2-(3,4-dimethoxyphenyl)ethanamide 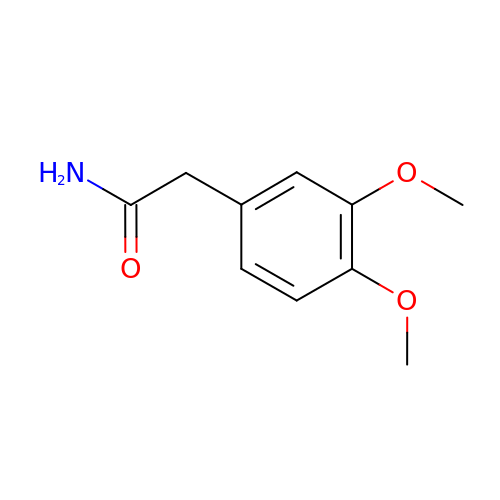| C10 H13 N O3 | CUWOZWFDSYIYHL-UHFFFAOYSA-N> GKRVLIVDDAAFMRMMLKDIITKAGYEVAGEATNGREAVEKYKELKPDIVTMDITMP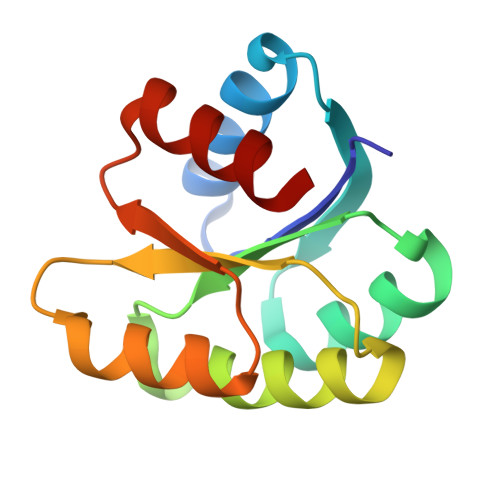EMNGIDAIKEIMKIDPNAKIIVCSAMGQQAMVIEAIKAGAKDFIVKPFQPSRVVEALNKVS[1-[2,4-bis(chloranyl)-3-(trifluoromethyl)phenyl]-1,2,3-triazol-4-yl]methanol | C10 H6 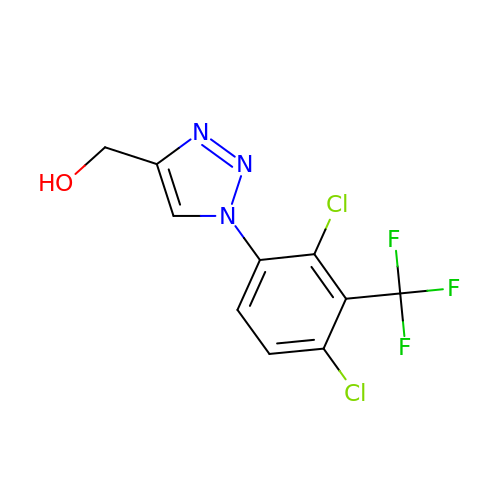Cl2 F3 N3 O | KVIREHNULVZQCY-UHFFFAOYSA-N> TDTTNSIKHVISPLARQTLQDRDLTRPVAGKRPIRLLPWLQVVKIGGRVMDRGADAILPLVEELRKLLPEHRLLILTGAGVRARHVFSVGLDLGLPVGSLAPLAASEAGQNGHILAAMLASEGVSYVEHPTVADQLAIHLSATRAVVGSAFPPYHHHEFPGSRIPPHRADTGAFLLADAFGAAGLTIVENVDGIYTADPNGPDRGQARFLPETSATDLAKSEGPLPVDRALLDVMATARHIERVQ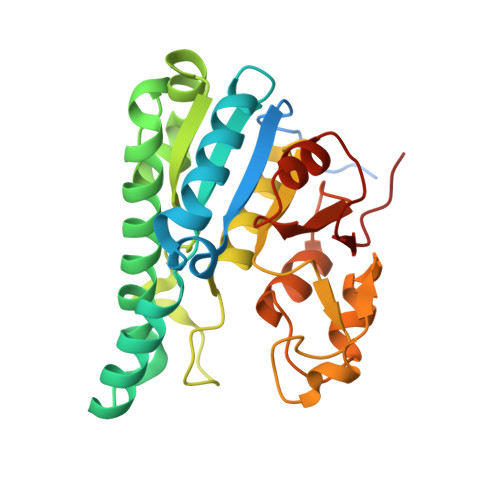VVNGLVPGRLTAALRGEHVGTLIRTGVRPA S-METHYL-METHIONINE | 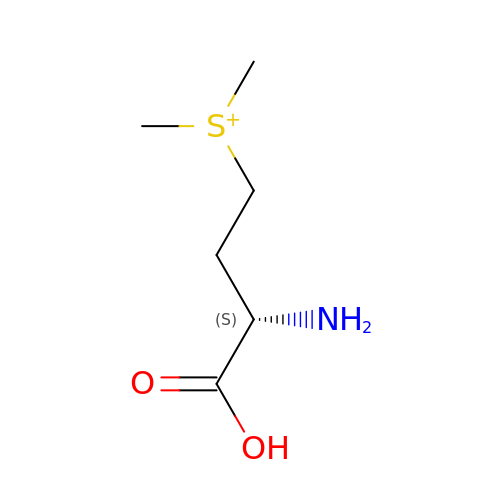C6 H14 N O2 S | YDBYJHTYSHBBAU-YFKPBYRVSA-O> SEQLVPIRLEFDQDRDRFFLRDTLLWNKNDKLIKIEDFVDDMLRDYRFEDATREQHIDTICQSIQEQIQEFQGNPYIELNQDRLGGDDLRIRIKL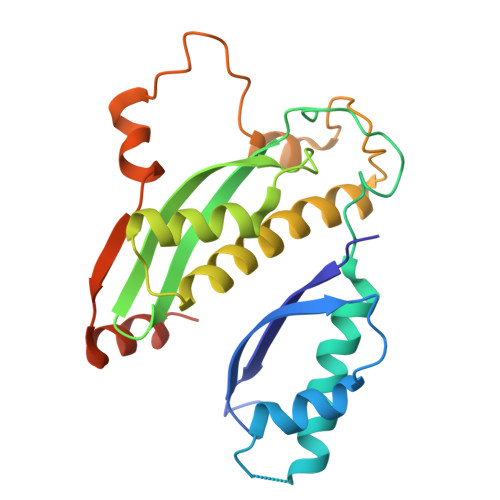DIVVGQNQLIDQFEWDISNSDNCPEEFAESMCQELELPGEFVTAIAHSIREQVHMYHKSLALLGYNFDGSAIEDDDIRSRMLPTITLDDVYRPAAESKIFTPNLLQISAAELERLDKDKDRDTRRKRRQGRS>MAHHHHHHSSGLEVLFQGPMNERFTLPAHSPALAALVPEFLDLARAASGDPAAEERDLAVWENLTEHVSLDYRFANPPVHGPGDWDTYDSRFVDPAGVEIGTLQGTGRILYERSSDAHLMMYYREQLTFPDGTAQTAGWVDGTAILGGAWQRFPILGSGGRYGSMIGLRSFQPTPEAPHSLYRTHLVLREIPGGHGLTDPEEIDAALSLLGAFVGPSVNPATGNGRLEPPVRAG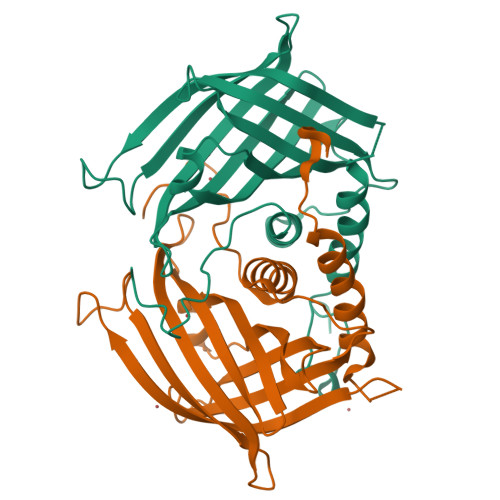RTA[4x]> GSHTAEEDMEDDTSWRSEATFQFTVERFSRLSESVLSPPCFVRNLPWKIMVMPRFYPDRPHQKSVGFFLQCNAESDSTSWS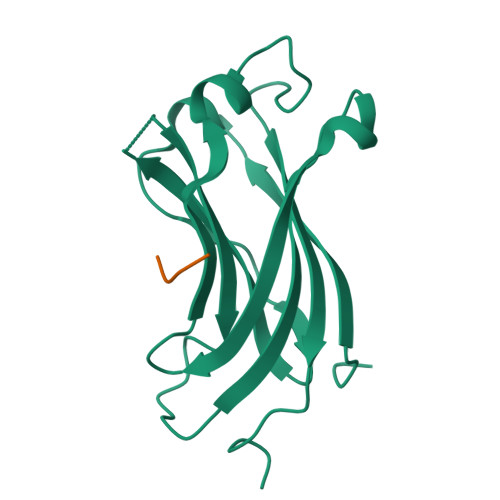CHAQAVLKIINYRDDEKSFSRRISHLFFHKENDWGFSNFMAWSEVTDPEKGFIDDDKVTFEVFVQADAPHGVAW;> LDLAHSSESQ>[2x]MAAAVVLAAGLRAARRAVAATGVRGGQVRGAAGVTDGNEVAKAQQATPGGAAPTIFSRILDKSLPADILYEDQQCLVFRDVAPQAPVHFLVIPKKPIPRISQAE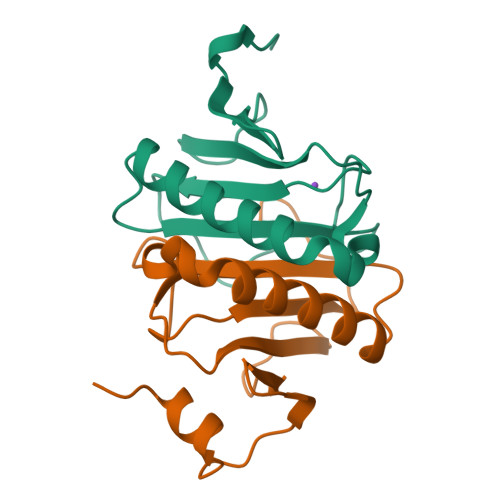EEDQQLLGHLLLVAKQTAKAEGLGDGYRLVINDGKLGAQSVYHLHIHVLGGRQLQWPPG> HDVGEVNGDALSAQEYQNLVEEYTEVIKLSRGVTALNDEQTNQVRDEVWRSYVNNKLVEKEAKALGLTVSAAEIQDILKAGVHPLLQQTPFRNPQTGAFDKDMLNKFLVDYAKMNESQMPAQYAEQYNNMYKYWSFIQKTLVQSRLAEKYQALVAKALLSNPVEAQDAFDARVNQYDLLMAAVPYSSIVDSTIVVKESELKDLYNKKKEQFKQYQESRDIKYIDVQVTASAEDRAAIQQEVDEATAQLATTTDDYTSFIRSVGSEAPYVDLFYNKTAFPSDVVARLDSASVGSVYGPYYNGADNTINSFKVVAKTAAADSIEFRQIQVFAEDALKTKALADSIYTAIKGGANFADLAKKYGQTGETNWMSSAQYEGAQIDGDNLKFISAINNTGVNEVVNLPLGQANVILQVTNKKAVKDKYKVAVVKREVEFSKETYNRAYNDFSQFIAANPTAEKMIANAEEAGYKLLDRRDLYSSEHTIGGVRGTKEALRWAFSAKPGDVSGLYECGESDHMVAVALVGVTP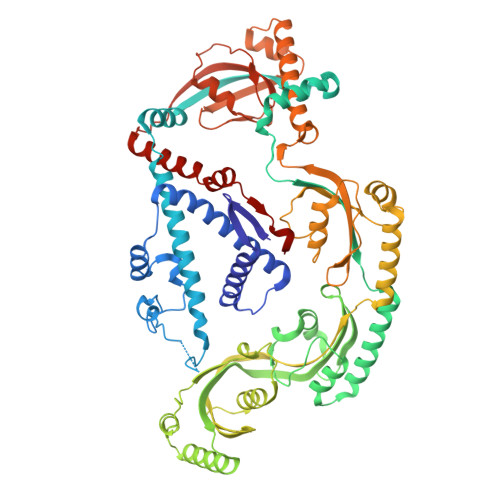EGYRPLKAVQDQLRAEIVKDKKAEKIMADMKAANATSLDQYKAMSGAVSDSLKLVTFAAPAYVSALRSSEPLVGAYASVAEMNKLSAPIKGNAGVFVLQMYGKDKLSDTFNAKDEEATLANMHARFASRLMNDLYLKGKVKDTRYLFF5-phenyltetrazolo[1,5-a]pyrimidin-7-ol | C10 H7 N5 O | 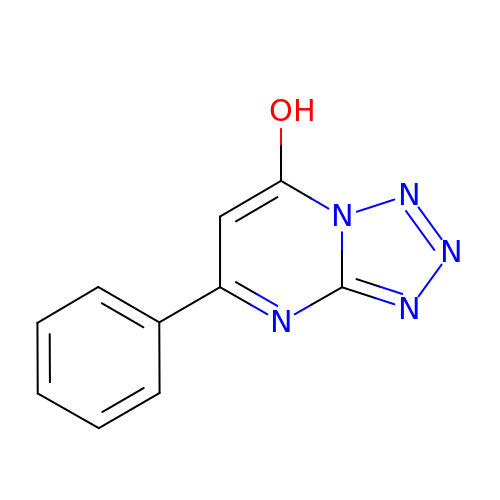ZEMGYOQXYFNSGE-UHFFFAOYSA-N>MTTPQIDERAMEAGAAALQETIVDPGPLDVTALAVAAALAAGLHSAADDPAAALDKCIVLDELTEFAEKLVVHDRPGGIGTTVEYVEVYEDASGVRLGTATGNAVVLKMEPHMWQFHQSVSELADGSFEAVGVIDCTAMLRRMTQVLR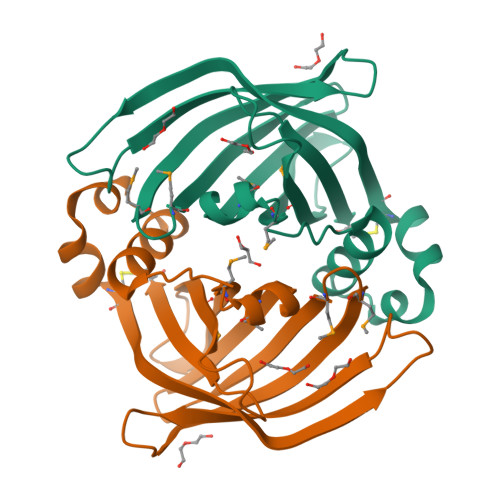VTGRSGRYAGKSGFMTLAISDPNQRPPHYSVQVVLC[2x]> MFVRKNPKSDKFKVKRFHHIEFWCGDATNVARRFSWGLGMRFSAKSDLSTGNMVHASYLLTSGDLRFLFTAPYSPSLSAGEIKPTTTASIPSFDHGSCRSFFSSHGLGVRAVAIEVEDAESAFSISVANGAIPSSPPIVLNEAVTIAEVKLYGDVVLRYVSY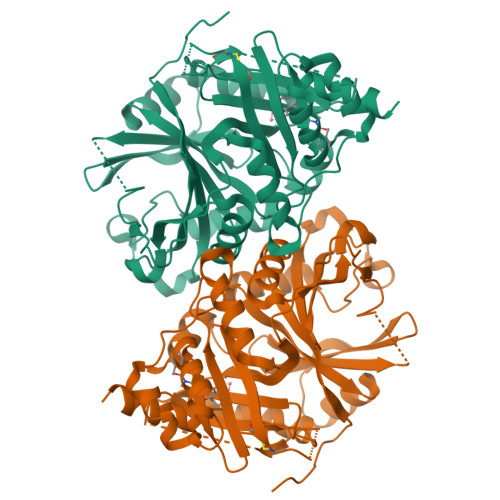KAEDTEKSEFLPGFERVEDASSFPLDYGIRRLDHAVGNVPELGPALTYVAGFTGFHQFAEFTADDVGTAESGLNSAVLASNDEMVLLPINEPVHGTKRKSQIQTYLEHNEGAGLQHLALMSEDIFRTLREMRKRSSIGGFDFMPSPPPTYYQNLKKRVGDVLSDDQIKECEELGILVDRDDQGTLLQIFTKPLGDRPTIFIEIIQRVGCMMKDEEGKAYQSGGCGGFGKGNFSELFKSIEEYEKTLEAKQLVG>HHHHHHMNRNPDQNTLPNITLKIIETYLGRVPSVNEYHMLKSQARNIQKITVFNKDIFVSLVKKNKKRFFSDVNTSASEIKDRILSYFSKQTQTYNIGKLFTIIELQSVLVTTYTDILGVLTIKAPNVISSKISYNVTSMEELARDMLNSMNVAVIDKAKVMGRHNVSSLVKNVNKLMEEYLRRHNKSCICYGSYSLYLINPNIRYGDIDILQTNSRTFLIDLAFLIKFITGNNIILSKIPYLRNYMVIKDENDNHIIDSFNIRQDTMNVVPKIFIDNIYIVDPTFQLLNMIKMFSQI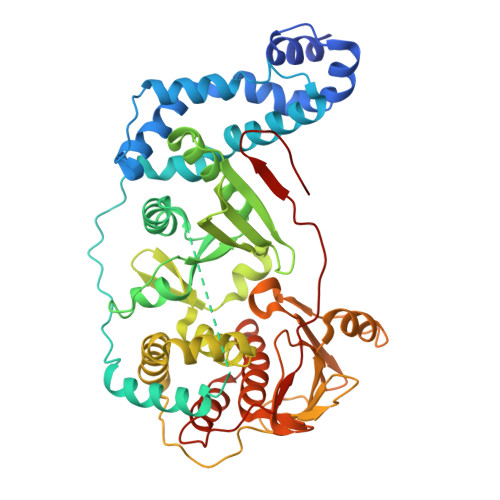DRLEDLSKDPEKFNARMATMLEYVRYTHGIVFDGKRNNMPMKCIIDENNRIVTVTTKDYFSFKKCLVYLDENVLSSDILDLNADTSCDFESVTNSVYLIHDNIMYTYFSNTILLSDKGKVHEISARGLCAHILLYQMLTSGEYKQCLSDLLNSMMNRDKIPIYSHTERDKKPGRHGFINIEKDIIVF[2x]> EFWYVEXEK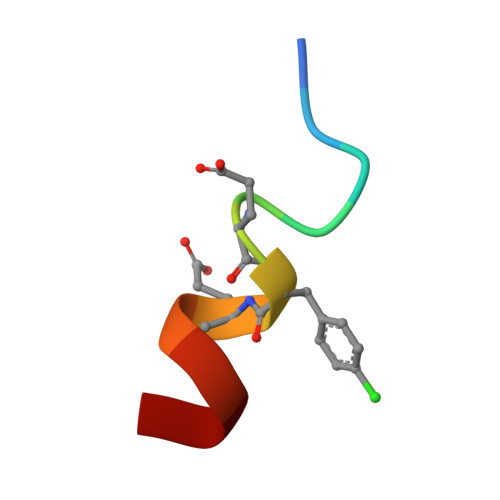LLR>MITTGKVWKFGDDISTDEITPGRYNLTKDPKELAKIAFIEVRPDFARNVRPGDVVVAGKNFGIGSSRESAALALKALGIAGVIAESFGRIFYRNAINIGIPLLLGKTEGLKDGDLVTVNWETGEVRKGDEILMFEPLEDFLLEIVREGGILEYIRRR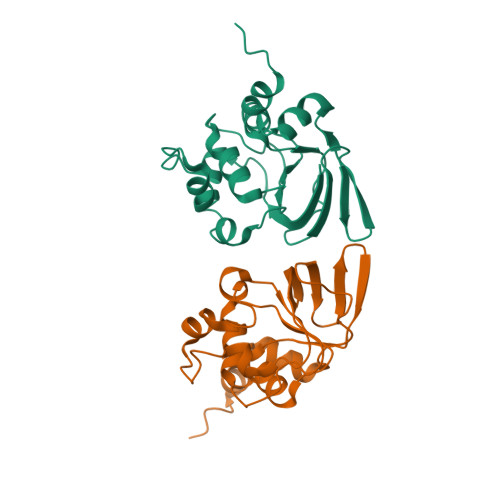GDLCIR[2x]>GSHMTELLKNHVAGQWIAGTGAGITLTDPVTGVALVRVSSEGLDLARAFSFAREDGGAALRALTYAQRAARLADIVKLLQAKRGDYYAIATANSGTTRNDSAVDIDGGIFTLSYYAKLGASLGEVHALRDGSAESLSKDRSFSAQHVLSPTRGVALFINAFNFPSWGLWAKAAPALLSGVPVIVKPATATAWLTQRMVADVVDAGILPPGALSIICGSSAGLLDQIRSFDVVSFTGSADTAATLRAHPAFVQRGARLNVEADSLNSAILCADATPDTPAFDLFIKEVVREMTVKSGQKCTAIRRAFVPEAALEPVLEALKAKLAKITVGNPRNDAVRMGSLVSREQYENVLAGIAALREEAVLAYDSSAVPLIDADANIAACVAPHL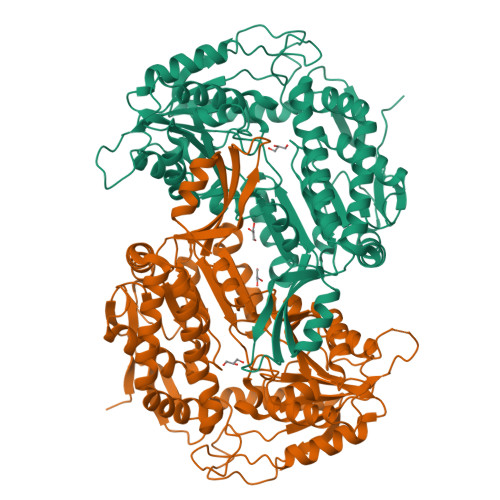FVVNDPDNATLLHDVEVFGPVASVAPYRVTTDTNALPEAHAVALARRGQGSLVASIYSNDDAHLGRLALELADSHGRVHAISPSVQHSQTGHGNVMPMSLHGGPGRAGGGEELGGLRALAFYHRRSAIQAASAAIGTLTQATHWPAA[2x]> MAHHHHHHMRGEDNMLVEMRTYRITAGKVPEFLKIYQDEGLGIITQYARLRGCWTQDSGTLNSVVFWWAYDDYSHRAAQRE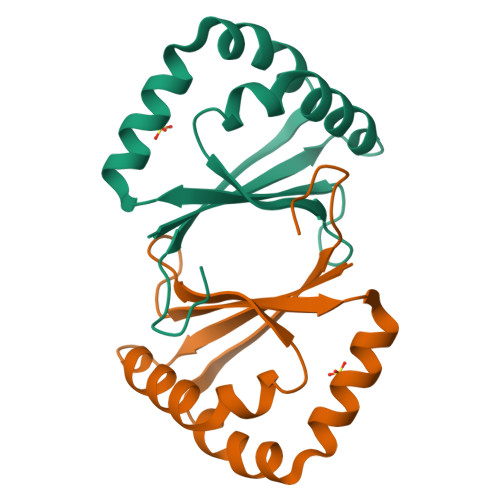RLAADPQWQAFTPRIVPYLEHQESVFLVPAAFCPDV>[2x]MEFTTGLMSLDTALNEMLSRVTPLTAQETLPLVQCFGRILASDVVSPLDVPGFDNSAMNGYAVRLADIASGQPLPVAGKSFAGQPYHGEWPAGTCIRIMTGAPVPEGCEAVVMQEQTEQMDNGVRFTAEVRSGQNIRRRGED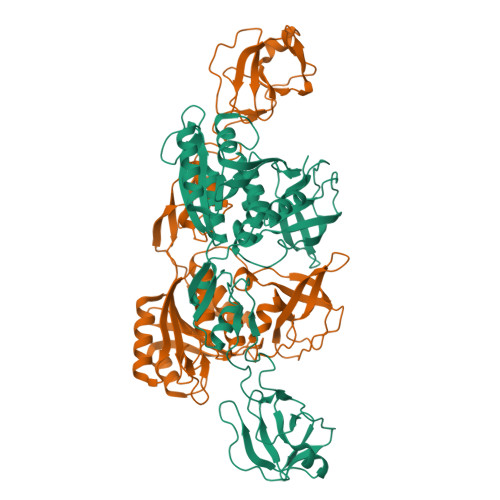ISAGAVVFPAGTRLTTAELPVIASLGIAEVPVIRKVRVALFSTGDELQLPGQPLGDGQIYDTNRLAVHLMLEQLGCEVINLGIIRDDPHALRAAFIEADSQADVVISSGGVSVGEADYTKTILEELGEIAFWKLAIKPGKPFAFGKLSNSWFCGLPGNPVSATLTFYQLVQPLLAKLSGNTASGLPARQRVRTASRLKKTPGRLDFQRGVLQRNADGELEVTTTGHQGSHIFSSFSLGNCFIVLERDRGNVEVGEWVEVEPFNALFGGL>[2x]HHHHHHMALQLAAHSDARSGPVGSNGGQFWSFRPVRPLNKIVLSFSGSPDQTLNLISITFSSNP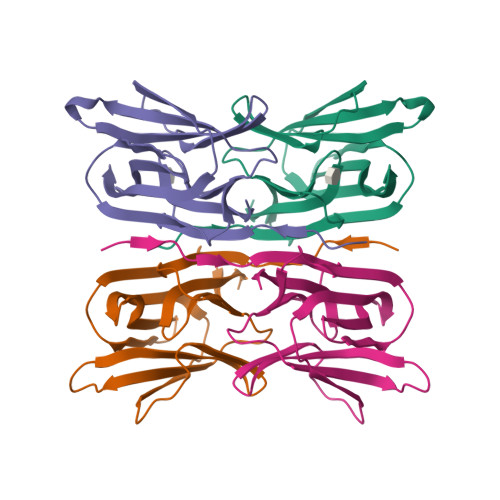TDIITVGGVGPEPLTYTETVNIDGDIIEISGMIANYKGYNVIRSIKFTTNKKEYGPYGANAGTPFNIKIPDGNKIVGFFGNSGWYVDAIGAYYTAK[3-(2-methylimidazol-1-yl)phenyl]methanamine | C11 H13 N3 | 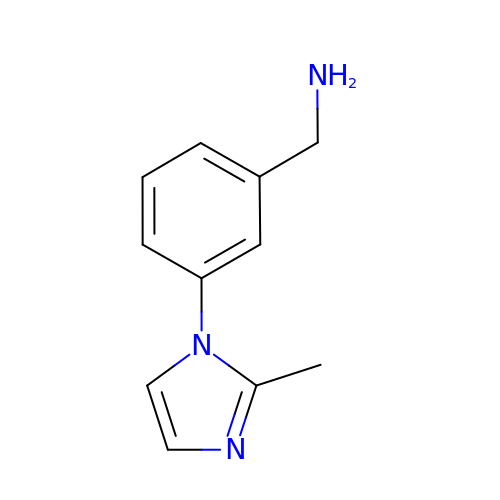CECWODAAUDOPCU-UHFFFAOYSA-N(2R,3R,4S,5R,6S)-2-(hydroxymethyl)-6-{[(2S,3R,4S,5S,6S)-3,4,5-trihydroxy-6-({[(1-{[(2R,3S,4S,5R,6S)-3,4,5-trihydroxy-6-methoxytetrahydro-2H-pyran-2-yl]methyl}-1H-1,2,3-triazol-4-yl)methyl]sulfanyl}methyl)tetrahydro-2H-pyran-2-yl]sulfanyl}tetrahydro-2H-pyran-3,4,5-triol 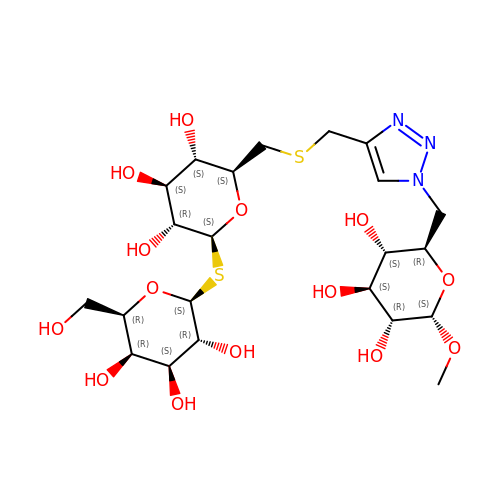(non-preferred name) | C22 H37 N3 O14 S2 | NRANZAMORPDRSV-CBEZMCEXSA-N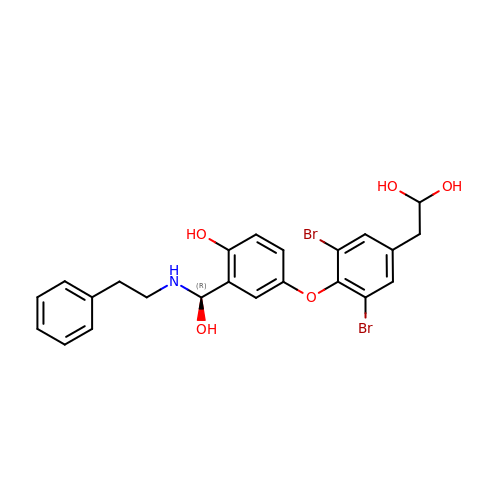2-[3,5-DIBROMO-4-(4-HYDROXY-3-{HYDROXY[(2-PHENYLETHYL)AMINO]METHYL}PHENOXY)PHENYL]ETHANE-1,1-DIOL | C23 H23 Br2 N O5 | KIRQJXNQGZAKGR-UHFFFAOYSA-N> MGSMLPLYLLTNAKGQQMQIELKNGEIIQGILTNVDNWMNLTLSNVTEYSEESAINSEDNAESSKAVKLNEIY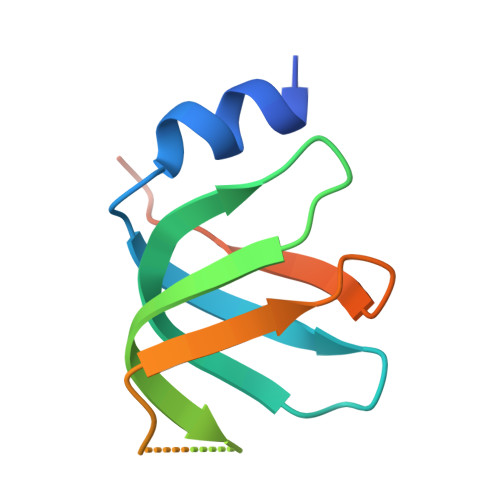IRGTFIKFIKLQDNIIDKVKQQI> GPMSETSFNLISEKCDILSILRDHPENRIYRRKIEELSKRFTAIRKTKGDGNCFYRALGYSYLESLLGKSREIFKFKERVLQTPNDLLAAGFEEHKFRNFFNAFYSVVELVEKDGSVSSLLKVFNDQSASDHIVQFLRLLTSAFIRNRADFFRHFIDEEMDIKDFCTHEVEPMATECDHIQITALSQALSIALQVEYVDEMDTALNHHVFPEAATPSVYLLYKTSHYNILYAADKH

Ubiquitin thioesterase OTUB2, a cysteine protease from the ovarian tumor (OTU) deubiquitinase superfamily, is often overexpressed during tumor progression and metastasis. Ovarian tumor (OTU) domain-containing ubiquitin aldehyde-binding protein 2 (OTUB2) is an active-site cysteine containing DUB. Recent research progress revealed that elevated OTUB2 expression correlates with tumorigenesis and metastasis. OTUB2 can promote tumorigenic progression of non-small cell lung cancer cells through deubiquitination of U2AF2, stimulation of the Warburg effect, and activation of AKT/mTOR signaling. Moreover, OTUB2 has been identified as a cancer stemness and metastasis-promoting factor that deubiquitinates YAP/TAZ proteins in breast cancer cells, whereby poly-SUMOylation on OTUB2 lysine 233 mediates the interaction with YAP/TAZ. These studies demonstrate OTUB2 to be a relevant therapeutic target, and the development of OTUB2-specific inhibitors can potentially be beneficial for cancer therapies.

Here, we describe the development of an improved OTUB2 inhibitor, LN5P45, comprising a chloroacethydrazide moiety that covalently reacts to the active-site cysteine residue. For our best inhibitor, LN5P45, we solved the X-ray co-crystal structure in complex with OTUB2, and we conducted a streamlined cysteine activity-based protein profiling (SLC-ABPP), which revealed that LN5P45 selectively engages endogenous OTUB2 over other ubiquitin machinery components. LC–MS analysis of OTUB2 before and after reaction with LN5P45 confirmed the formation of a covalent complex by showing a mass difference of 230 Da, which corresponds to a substitution reaction at the chloride. The phenyl ring moiety points outside the protein toward the solvent and has as such no obvious interactions; there are no aromatic protein residues or arginine around the active site that could π–π stack with the phenyl moiety of LN5P45. The trans orientation on the other hand nicely positions the inhibitor inside the small groove leading to the active site. The carbonyl directly attached to the cyclopropane ring interacts with the side chain of His224 through a hydrogen bond, and the Glu174 side chain carboxylate also forms hydrogen bonds with both of the hydrazide amines. We determined the preferred absolute stereochemistry as (1S,2S), and the LN5P45-OTUB2 co-crystal structure explained the molecular details of the inhibitor binding mode.As the most abundant viral protein encoded by the M gene segment, matrix protein 1 (M1) forms a shell underneath a host cell-derived lipid biolayer to connect the vRNPs with the viral envelope in mature virions. The full-length M1 protein includes 252 amino acids consisting of a highly organized N-terminal domain and a flexible but less ordered C-terminal domain that are linked by a protease-sensitive loop. So far, only the N-terminal domain of M1 has been structurally resolved at an atomic level, showing that at neutral pH the physiological monomers have a high tendency to oligomerize via a so-called ‘face-to-back’ arrangement, whereas at acidic pH the N-terminal domain exists as a dimeric structure in a so-called ‘face-to-face’ arrangement.

However, the G88E mutation causes M1 to be trapped in a face-to-face orientation regardless of pH that consequently resulted in inefficient virus growth and genetic instability. Surprisingly, M(NLS-88E)-neutral dimerizes in a face-to-face manner at neutral pH in contrast to a face-to-back monomer–monomer arrangement as possessed by wt-M11EA3 (pH 7.0) and M(NLS-88R)-neutral. A further look at M(NLS-88E)-neutral structure reveals that the G88E mutation results in three inter-subunit salt-bridge/hydrogen-bond interactions including Lys104-NZ to Glu88-OE1 (and its symmetry-related counterpart) and Arg134-NE to Glu88-OE2 that may explain why M(NLS-88E)-neutral that is predicted to crystallize as monomers in a face-to-back arrangement is actually driven to dimerize in a face-to-face manner at neutral pH. Interactions between the monomers that form the face-to-face dimer in M(NLS-88R)-acidic, M(NLS-88E)-acidic or M(NLS-88E)-neutral involve hydrophobic contacts (mainly between the symmetry-related helices H6, and between helices H9 and loops L9), as well as several hydrogen-bond and/or salt-bridge interactions. However, M(NLS-88E) M1 is trapped in a face-to-face-oriented conformation irrespective of environmental pH. In the case of M(NLS-88E)-neutral with misshapen face-to-face monomer–monomer interactions that seem unfavorable for M1 oligomerization, a thin, uneven and broken M1 layer still forms beneath the M(NLS-88E) viral envelope as exhibited in our TEM images. This could be due to the presence of the C terminus that may provide sufficient stabilization for a malformed M1 layer.

>MHHHHHHSLLTEVETYVLSIVPSGPLKAEIAQRLEDVFAGKNTDLEVLMEWLKTRPILSPLTKGILGFVFTLTVPSERGLQRRRFVQNALNGNEDPNNMDKAVKLYSKLKSEITFHGAKEIALSYSAGALASCMGLIYNRMGAVTTEVAFGLVCATCEQIADSQHRSHRQM[2x]> GSHMAPFVAKDIRVDGVQGDLEQQIRASLPVRAGQRVTDNDVANIVRSLFVSGRFDDVKAHQEGDVLVVSVVAKSIISDVKIKGNSIIPTEALKQNLDANGFKVGDVLIREKLNEFAKSVKEHYASVGRYNATVEPIVNTLPNNRAEILIQINEDDKAKLASLTFKGNESVSSSTLQEQMELQPDSWWKLWGNKFEGAQ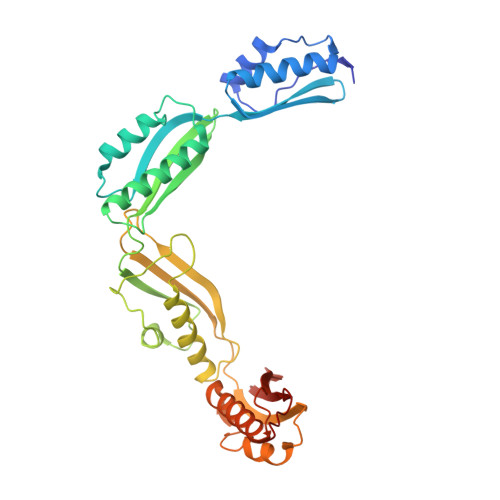FEKDLQSIRDYYLNNGYAKAQITKTDVQLNDEKTKVNVTIDVNEGLQYDLRSARIIGNLGGMSAELEPLLSALHLNDTFRRSDIADVENAIKAKLGERGYGSATVNSVPDFDDANKTLAITLVVDAGRRLTVRQ>MSERLSITPLGPYIGAQISGADLTRPLSDNQFEQLYHAVLRHQVVFLRDQAITPQQQRALAQRFGELHIHPVYPHAEGVDEIIVLDTHNDNPPDNDNWHTDVTFIETPPAGAILAAKELPSTGGDTLWTSGIAAYEALSVPFRQLLSGLRAEHDFRKSFPEYKYRKTEEEHQRWREAVAKNPPLLHPVVRTHPVSGKQALFVNEGFTTRIVDVSEKESEALLSFLFAHITKPEFQVR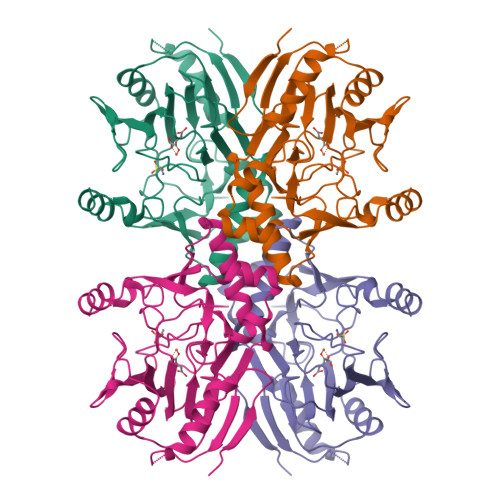WRWQPNDIAIWDNRVTQHYANADYLPQRRIMHRATILGDKPFYRAG[2x]>ESHMAMDLGGYLTRIGLDGRPRPDLGTLHAIVAAHNRSIPFENLDPLLGIPVADLSAEALFAKLVDRRRGGYCYEHNGLLGYVLEELGFEVERLSGRVVWMRADDAPLPAQTHNVLSVAVPGADGRYLVD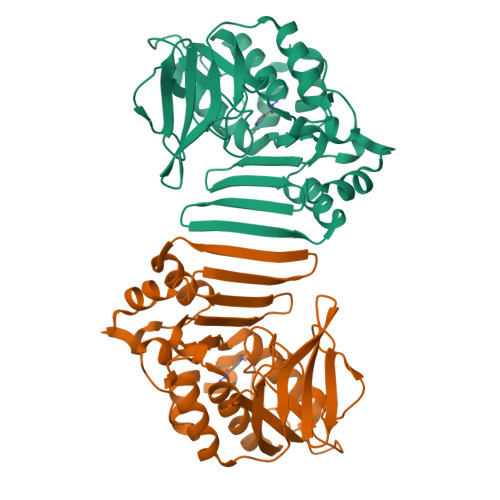VGFGGQTLTSPIRLEAGPVQQTRHEPYRLTRHGDDHTLAAQVRGEWQPLYTFTTEPRPRIDLEVGSWYVSTHPGSHFVTGLTVAVVTDDARYNLRGRNLAVHRSGATEHIRFDSAAQVLDAIVNRFGIDLGDLAGRDVQARVAEVLDT[4x]>[2x]AATYAQTLQNIPETNVTTLDNGLRVASEESSQPTCTVGVWIGAGSRYENEKNNGAGYFVEHLAFKGTKKRPCAAFEKEVESMGAHFNGYTSREQTAFYIKALSKDMPKVVELLADVVQNCALEESQIEKERGVILQELKEMDNDMTNVTFDYLHATAFQGTALARTVEGTTENIKHLTRADLASYIDTHFKAPRMVLAAAGGISHKELVDAARQHFSGVSFTYKEDAVPILPRCRFTGSEIRARDDALPVAHVALAVEGPGWADPDNVVLHVANAIIGRYDRTFGGGKHLSSRLAALAVEHKLCHSFQTFNTSYSDTGLFGFHFVADPLSIDDMMFCAQGEWMRLCTSTTESEVKRAKNHLRSAMVAQLDGTTPVCETIGSHLLNYGRRISLEEWDSRISAVDARMVRDVCSKYIYDKCPALAAVGPIEQLLDYNRIRSGMYWIRF;>[2x]SLKVAPKVAVSAAAERVKLCPGAEDLEITKLPNGLIIASLENFSPASRIGVFIKAGSRYETTANLGTAHLLRLASPLTTKGASSFRITRGIEAVGGSLSVYSTREKMTYCVECLRDHVDTVMEYLLNVTTAPEFRPWEVTDLQPQLKVDKAVAFQSPQVGVLENLHAAAYKTALANPLYCPDYRIGKITSEQLHHFVQNNFTSARMALVGIGVKHSDLKQVAEQFLNIRSGAGTSSAKATYWGGEIREQNGHSLVHAAVVTEGAAVGSAEANAFSVLQHVLGAGPLIKRGSSVTSKLYQGVAKATTQPFDASAFNVNYSDSGLFGFYTISQAAHAGEVIRAAMNQLKAAAQGGVTEEDVTKAKNQLKATYLMSVETAQGLLNEIGSEALLSGTHTAPSVVAQKIDSVTSADVVNAAKKFVSGKKSMAASGDLGSTPFLDEL;>[2x]MAPNIRKSHPLLKMINNSLIDLPAPSNISAWWNFGSLLAVCLMTQILTGLLLAMHYTADTSLAFSSVAHTCRNVQYGWLIRNLHANGASFFFICIFLHIGRGLYYGSYLYKETWNTGVILLLTLMATAFVGYVLPWGQMSFWGATVITNLFSAIPYIGHTLVEWAWGGFSVDNPTLTRFFALHFLLPFAIAGITIIHLTFLHESGSNNPLGISSDSDKIPFHPYYSFKDILGLTLMLTPFLTLALFSPNLLGDPENFTPANPLVTPPHIKPEWYFLFAYAILRSIPNKLGGVLALAASVLILFLIPFLHKSKQRTMTFRPLSQTLFWLLVANLLILTWIGSQPVEHPFIIIGQMASLSYFTILLILFPTIGTLENKMLNY;>[2x]GELELHPPAFPWSHGGPLSALDHSSVRRGFQVYKQVCSACHSMDYVAFRNLIGVTHTEAEAKALAEEVEVQDGPDENGELFMRPGKISDYFPKPYPNPEAARAANNGALPPDLSYIVNARHGGEDYVFSLLTGYCDPPAGVVVREGLHYNPYFPGQAIGMAPPIYNEILEYDDGTPATMSQIAKDVCTFLRWAAEPEHDQRKRMGLKMLLISALLTSLLYYMKRHKWSVLKSRKMAYRPPK;>[2x]VHNDVTVPDFSAYRREDVMDATTSSQTSSEDRKGFSYLVTATACVATAYAAKNVVTQFISSLSASADVLALSKIEIKLSDIPEGKNVAFKWRGKPLFVRHRTQAEINQEAEVDVSKLRDPQHDLDRVKKPEWVILVGVCTHLGCVPIANSGDFGGYYCPCHGSHYDASGRIRKGPAPYNLEVPTYQFVGDDLVVVG;>[2x]AARATVAGGGRLMDRIRKWYYNAAGFNKYGLMRDDTLYEDDDVKEALKRLPKDLYNERMFRIKRALDLSLKHRILPKEQWVKYEEDKPYLEPYLKEVIRERLEREAWNKK;>[2x]GIHFGNLARVRHIITYSLSPFEQRAIPNIFSDALPNVWRRFSSQVFKVAPPFLGAYLLYSWGTQEFERLKRKNPADYENDQ;>[2x]LRGSGEEEEEELVDPLTTIREHCEQTEKCVKARERLELCDARVSSRSHTEEQCTEEL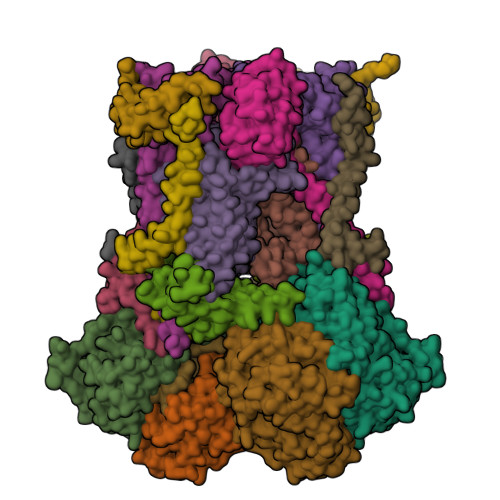FDFLHARDHCVAHKLFNKLK;>[2x]ALLRQAYSALFRRTSTFALTVVLGAVLFERAFDQGADAIFEHLNEGKLWKHIKHKYEASEE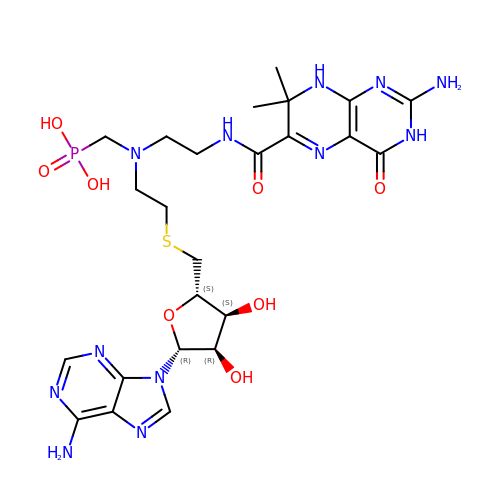5'-S-{2-[{2-[(2-amino-7,7-dimethyl-4-oxo-3,4,7,8-tetrahydropteridine-6-carbonyl)amino]ethyl}(phosphonomethyl)amino]ethyl}-5'-thioadenosine | C24 H35 N12 O8 P S | LNONYTMYGAJODO-HUYKWJOFSA-N1-(4-METHOXYPHENYL)METHANAMINE | C8 H11 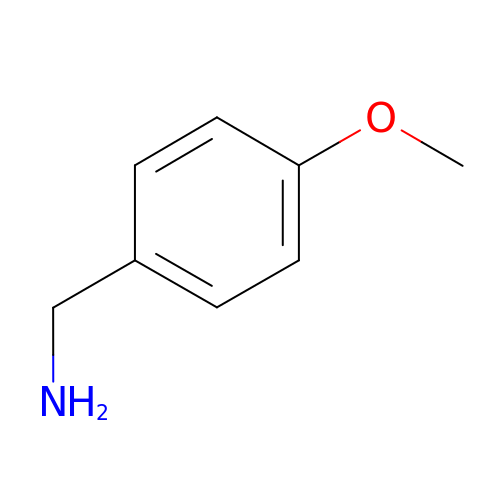N O | IDPURXSQCKYKIJ-UHFFFAOYSA-N> AVSLDR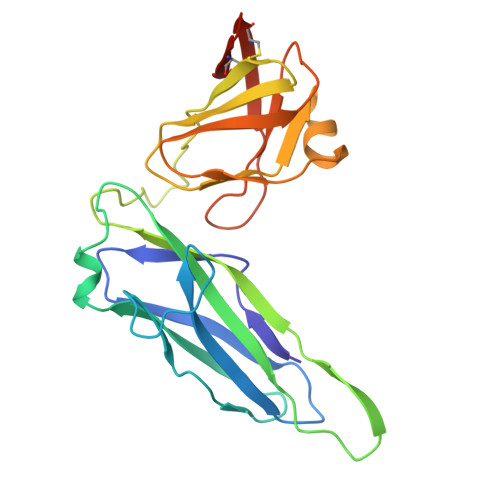TRAVFDGSEKSMTLDISNDNKQLPYLAQAWIENENQEKIITGPVIATPPVQRLEPGAKSMVRLSTTPDISKLPQDRESLFYFNLREIPPRSEKANVLQIALQTKIKLFYRPAAIKTRPNEVWQDQLILNKVSGGYRIENPTPYYVTVIGLGGSEKQAEEGEFETVMLSPRSEQTVKSANYNTPYLSYINDYGGRPVLSFICNGSRCSVKHHHHHH> MTKTLPKDFIFGGATAAYQAEGATHTDGKGPVAWDKYLEDNYWYTAEPASDFYHKYPVDLELAEEYGV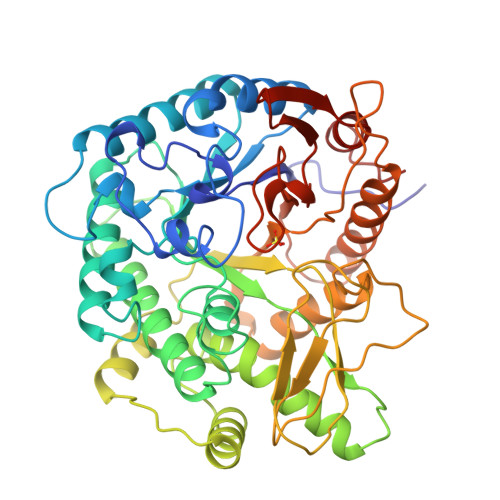NGIRISIAWSRIFPTGYGEVNEKGVEFYHKLFAECHKRHVEPFVTLHHFDTPEALHSNGDFLNRENIEHFIDYAAFCFEEFPEVNYWTTFNEIGPIGDGQYLVGKFPPGIKYDLAKVFQSHHNMMVSHARAVKLYKDKGYKGEIGVVHALPTKYPYDPENPADVRAAELEDIIHNKFILDATYLGHYCDKTMEGVNHILAENGGELDLRDEDFQALDAAKDLNDFLGINYYMSDWMQAFDGETEIIHNGKGEKGSSKYQIKGVGRRVAPDYVPRTDWDWIIYPEGLYDQIMRVKNDYPNYKKIYITENGLGYKDEFVDNTVYDDGRIDYVKQHLEVLSDAIADGANVKGYFIWSLMDVFSWSNGYEKRYGLFYVDFDTQERYPKKSAHWYKKLAETQVIE>ASYINAAFRSSRAYEVYFFECNKYVRVYYTPGKTDDKILTNLRLISSGFPS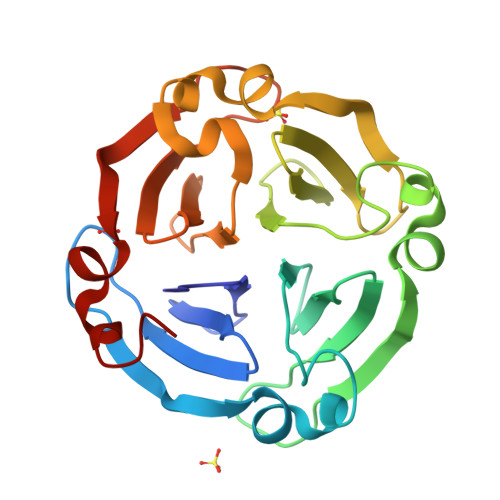LAGTAFAEPGIDCSFDTEASEAYVFSGSQCAYIDYAPGTTNDKILSGPTTIAEMFPVLKNTVFEDGIDSAFRSTKGKEVYLFKGNKYGRIAYDSKQLVGTIRNITDGFPVLKGTIFESGIDASFASHKEPEAYLFKGAQYVRIKFTPGATNNTLTGKVRPILDGWPCLRDILPT[3x]>MPLVSMTEMLNKAKAEGYAVGQFNLNNLEFTQAILLAAEEEKSPVILGVSEGAGRYMGGFKTVVNMVKGLMEDYKITVPVAIHLDHGSSFEKCKEVIDAGFTSVMIDASHHPFEENVEVTKKVVEYAHARGVSVEAELGTVGGQEDDVIADGVIYADPKECEELVKRTGIDCLAPALGSVHGPYKGEPNLGFKEMEEIGRITGVPLVLHGGTGIPTKDIQRAISLGTAKINVNTENQIASAKKVREVLAENPNMYDPRKYLGPARDAIKETV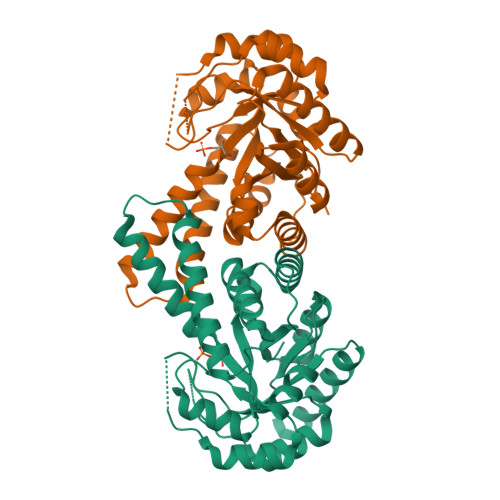IGKMREFGSSGKA[2x]>[6x]MINVDGEYLKIFAGRIKLMKAVILAAGLGTRLGGVPKPLVRVGGCEIILRTMKLLSPHVSEFIIVASRYADDIDAFLKDKGFNYKIVRHDRPEKGNGYSLL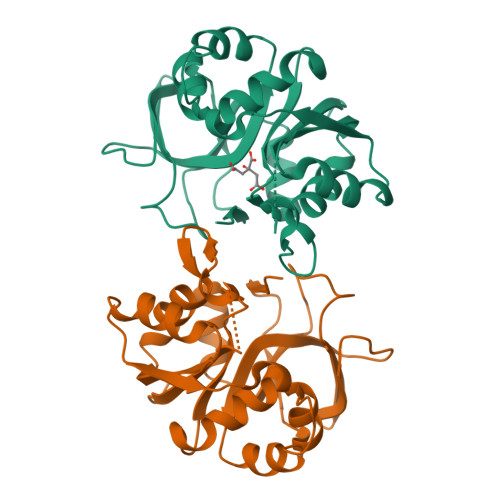VAKNHVEDRFILTMGDHVYSQQFIEKAVRGEGVIADREPRFVDIGEATKIRVEDGRVAKIGKDLREFDCVDTGFFVLDDSIFEHAEKLRDREEIPLSEIVKLARLPVTYVDGELWMDVDTKEDVRRANRAL>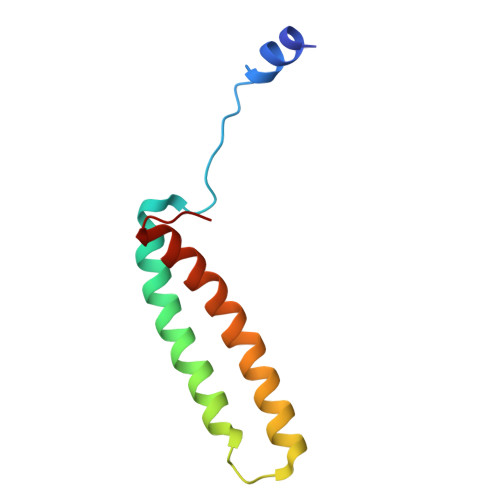 MTYEQLYKEFHSSKSFQPFIHLDTQPKFAICGLIVTLAVLSSALFAVGSKSSYIKKLFFYTILSVIGSLFAGLTTVFASNSFGVYV> HHHHHHSQDPNALIDRLGIQLKDNLVFSLGVESDKIKDL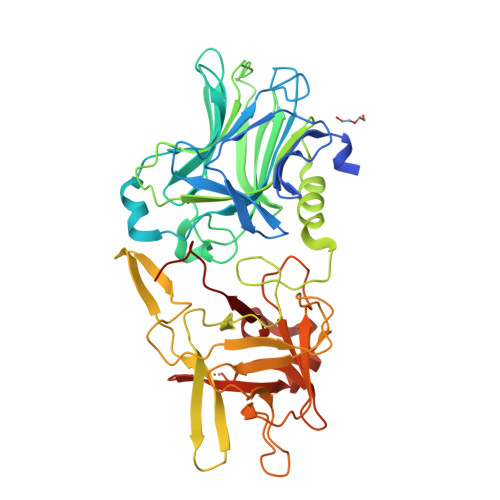SGNNTNLEVKTGVQIVDGRDSKTIRLNSNENSSIIVQKNESINFSYFSDFTISFWIRVPRLNKNDFIDLGIEYDLVNNMDNQGWKISLKDGNLVWRMKDRFGKIIDIITSLTFSNSFIDKYISSNIWRHITITVNQLKDCTLYINGDKIDSKSINELRGIDNNSPIIFKLEGNRNKNQFIRLDQFNIYQRALNESEVEMLFNSYFNSNILRDFWGEPLEYNKSYYMINQAILGGPLRSTYKSWYGEYYPYISRMRTFNVSSFILIPYLYHKGSDVEKVKIINKNNVDKYVRKNDVADVKFENYGNLILTLPMYSKIKERYMVLNEGRNGDLKLIQLQSNDKYYCQIRIFEMYRNGLLSIADDENWLYSSGWYLYSSGWYLDNYKTLDLKKHTKTNWYFVSEDEGWKE>SDLAREITPVNIEEELKSSYLDYAMSVIVGRALPDVRDGLKPVHRRVLYAMNVLGNDWNKAYKKSARVVGDVIGKYHPHGDSAVYDTIVRMAQPFSLRYMLVDGQGNFGSIDGDSAAAMRYTEIRLAKIAHELMADLEKETVDFVDNYDGTEKIPDVMPTKIPNLLVNGSSGIAVGMATNIPPHNLTEVINGCLAYIDDEDISIEGLMEHIPGPDFPTAAIINGRRGIEEAYRTGRGKVYIRARAEVEVDAKTGRETIIVHEIPYQVNKARLIEKIAELVKEKRVEGISALRDESDKDGMRIVIEVKRDAVGEVVLNNLYSQTQLQVSFGINMVALHHGQPKIMNLKDIIAAFVRHRREVVTRRTIFELRKARDRAHILEALAVALANIDPIIELIRHAPTPAEAKTALVANPWQLG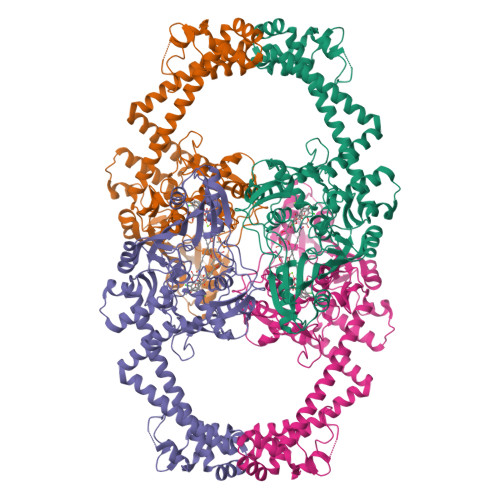NVAAMLERAGDDAARPEWLEPEFGVRDGLYYLTEQQAQAILDLRLQKLTGLEHEKLLDEYKELLDQIAELLRILGSADRLMEVIREELELVREQFGDKRRTEITA[2x]> GPKVPESGSMNLAAAERKKTGDLSVRSLHDIVKPEDFVLNSEHLTTVLVAVPKSLKSDFEKSYETLSKNVVPASASVIAEDAEYVLFNVHLFKKNVQEFTTAAREKKFIPREFNYSEELIDQLKKEHDSA;> MSSAITALTPNQVNDELNKMQAFIRKEAEEKAKEIQLKADQEYEIEKTNIVRNETNNIDGNFKSKLKKAMLSQQITKSTIANKMRLKVLSAREQSLDGIFEETKEKLSGIANNRDEYKPILQSLIVEALLKLLEPKAIVKALERDVDLIESMKDDIMREYGEKAQRAPLEEIVISNDYLNKDLVSGGVVVSNASDKIEINNTLEERLKLLSEEALPAIRLELYGPSKTRKFFD;> GPKVPMSQKNGIATLLQAEKEAHEIVSKARKYRQDKLKQAKTDAAKEIDSYKIQKDKELKEFEQKNAGGVGELE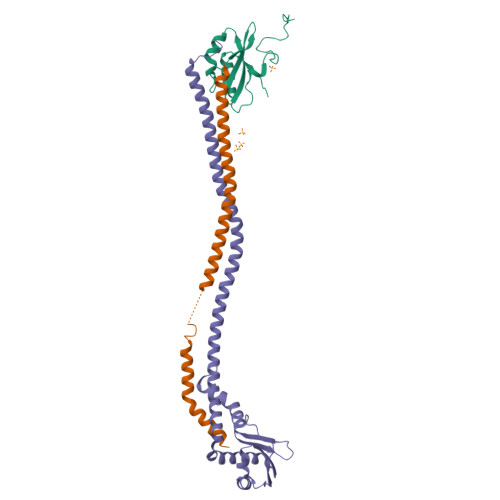KKAEAGVQGELAEIKKIAEKKKDDVVKILIETVIKPSAEVHINAL> GSEAAGGEQRELLIQRLRAAVHYTTGALAQDVAEDKGVLFSKQTVAAISEITFRQAENFARDLEMFARHAKRSTITSEDVKLLARRSNSLLKYIT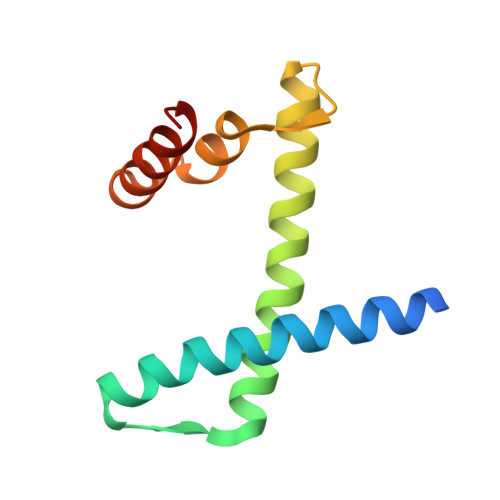QKSDELASSNME2-(3-bromophenoxy)-N-[(1S,2S,3R,5S)-2-hydroxybicyclo[3.1.0]hexan-3-yl]acetamide 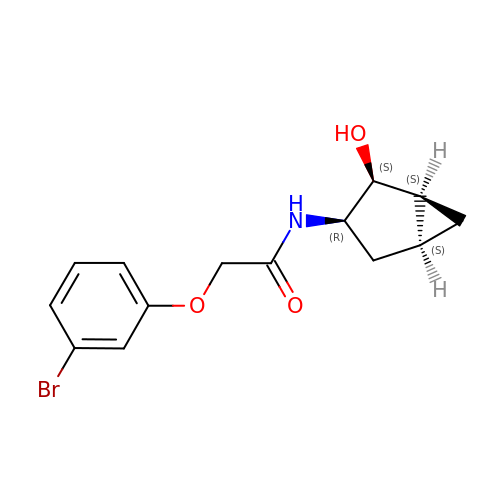| C14 H16 Br N O3 | ZHUQGQJYDVDPGM-GJBBRRBDSA-N> GPLGSPLTASMLASAPPQEQKQMLGERLFPLIQAMHPT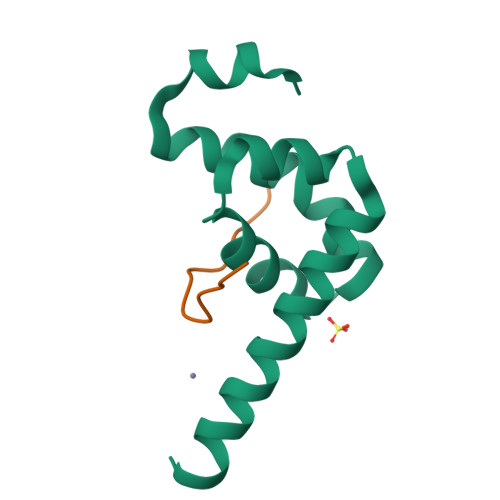LAGKITGMLLEIDNSELLHMLESPESLRSKVDEAVAVLQAHQAKEAAQKA;> RQLNVNAKPFVPNVH> MTCWLRGVTATFGRPAEWPGYLSHLCGRSAAMDLGPMRKSYRGDREAFEETHLTSLDPVKQFAAWFEEAVQCPDIGEANAMCLATCTRDGKPSARMLLLKGFGKDGFRFFTNFESRKGKELDSNPFASLVFYWEPLNRQVRVEGPVKKLPEEEAECYFHSRPK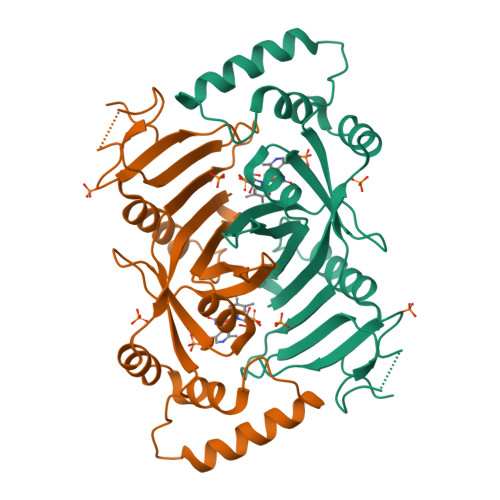SSQIGAVVSHQSSVIPDREYLRKKNEELEQLYQDQEVPKPKSWGGYVLYPQVMEFWQGQTNRLHDWIVFRRGLPTGDSPLGPMTHRGEEDWLYERLAP>MIVTTTSGIQGKEIIEYIDIVNGEAIMGANIVRDLFASVRDVVGGRAGSYESKLKEARDIAMDEMKELAKQKGANAIVGVD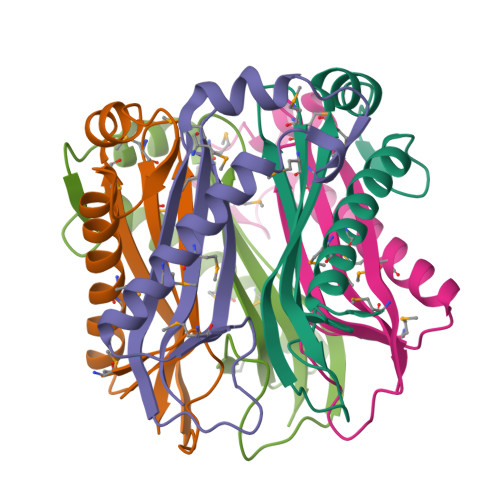VDYEVVRDGMLMVAVSGTAVRILEHHHHHH[5x]>[2x]MLSFLRSTGRPERRRASLPALLLFTAALVASGLTAAPAAQAADNPYQRGPDPTNASIEAATGPFAVGTQPIVGASGFGGGQIYYPTDTSQTYGAVVIVPGFISVWAQLAWLGPRLASQGFVVIGIETSTITDLPDPRGDQALAALDWATTRSPVRSRIDRTRLAAAGWSMGGGGLRRAACQRPSLKAIVGMAPWNTEKNWSCVTVPTLFFGGSSDAVASPNDHAKPFYNSITRAEKDYIELCNADHFFPTSANTTMAKYFISWLKRWVDNDTRYTQFLCPGPSTGLFAPVCASMNTCPFLEHHHHHH

In the present study, we report a PET hydrolase from Cryptosporangium aurantiacum (CaPETase) that exhibits remarkable PET degradation activity at ambient temperatures and high thermostability. CaPETase shows an α/β hydrolase fold and a nine-stranded β-sheet at the center surrounded by six α-helices and two 310-helices. Formation of one conserved disulfide bond (DS, C279/C297) and lack of an extended loop in the substrate binding site of CaPETase suggest that the enzyme originated from an ancestor of TfCut2 and LCC rather than IsPETase.

The G196T mutation resulted in positive effects on both thermostability and enzyme activity; thus, we finally generated CaPETaseDS2/DS4/NC1/NC4/HP1/SC2/G196T (CaPETaseM9) by integrating the G196T mutation into CaPETaseM8. CaPETaseM9 exhibited a Tm value of 83.2 °C, which corresponds to a 16.7 °C increase in Tm compared with CaPETaseWT. CaPETaseM9 showed much higher activity at all temperature conditions from 30 to 70 °C, and particularly, showed 41.7-fold higher specific activity at 60 °C than CaPETaseWT. To provide structural insights into the enhanced PET-degrading capacity of CaPETaseM9, we determined its crystal structure at a resolution of 1.53 Å. The formation of the introduced DS2 and DS4 disulfide bonds was clearly observed in CaPETaseM9, and the S–S interatomic length of both disulfide bonds was within the optimal disulfide bond length range. The side chain of the mutated V129T was flipped to form a hydrogen bond with the adjacent T131 and D132 residues, thereby further stabilizing the β4–α3 connecting loop. With respect to R198K, the mutated lysine residue moved inward to form hydrogen bonds with the main chains of N195 and D222, thereby stabilizing the wobbly tryptophan-containing loop. The mutated G196T formed a water-mediated hydrogen bond with the adjacent N195 residue, resulting in further stabilization of the wobbly tryptophan-containing loop. The A155R mutation changed the hydrophobic surface to a positive charge, which seems to increase the attachment of the enzyme to the PET surface, as suggested by a previous report. Finally, the N109A mutation appeared to strengthen internal hydrophobic interactions.> MAYHKKVVDHYENPRNVG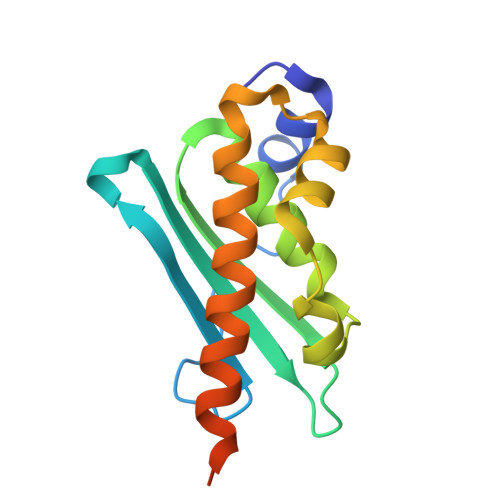SLDKTSKNVGTGLVGAPACGDVMKLQIQVDEKGKIVDARFKTFGCGSAIASSSLATEWVKGKTVEEALTIKNTDIAKELCLPPVKLHCSILAEDAIKAALADYKLKQEPKKGEAEKKLEHHHHHH>[2x]GEEQMRLPSADVYRFAEPDSEENIIFEENMQPKAGIPIIKAGTVIKLIERLTYHMYADPNFVRTFLTTYRSFCKPQELLSLIIERFEIPEPEPTEADRIAIENGDQPLSAELKRFRKEYIQPVQLRVLNVCRHWVEHHFYDFERDAYLLQRMEEFIGTVRGKAMKKWVESI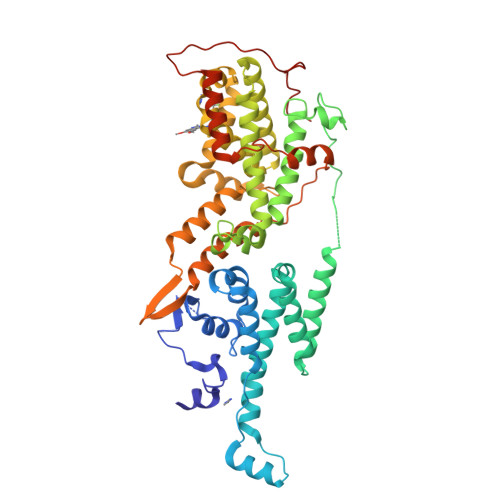TKIIQRKKIARDNGPGHNITFQSSPPTVEWHISRPGHIETFDLLTLHPIEIARQLTLLESDLYRAVQPSELVGSVWTKEDKEINSPNLLKMIRHTTNLTLWFEKCIVETENLEERVAVVSRIIEILQVFQELNNFNGVLEVVSAMNSSPVYRLDHTFEQIPSRQKKILEEAHELSEDHYKKYLAKLRSINPPCVPFFGIYLTNILKTEEGNPEVLKRHGKELINFSKRRKVAEITGEIQQYQNQPYCLRVESDIKRFFENLNPMGNSMEKEFTDYLFNKSLEIEPRNPKPLPRFPKKYSYPLKSPGVRPSNPRPGT>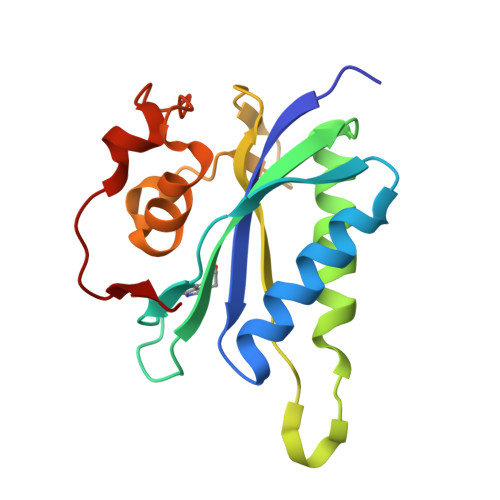[2x]GSHMIQAYLGLGSNIGDRESQLNDAIKILNEYDGISVSNISPIYETAPVGYTEQPNFLNLCVEIQTTLTVLQLLECCLKTEECLHRIRKERWGPRTLDVDILLYGEEMIDLPKLSVPHPRMNERAFVLIPLNDIAANVVEPRSKLKVKDLVFVDDSVKRYK>TYQYNMNFEKLGKCIIINNKNFDKVTGMGVRNGTDKDAEALFKCFRSLGFDVIVYNDCSCAKMQDLLKKASEEDHTNAACFACILLSHGEENVIYGKDGVTPIKDLTAHFRGDRCKTLLEKPKLFFIQACRGTELDDGIQADSGPINDTDANPRYKIPVEADFLFAYSTVPGYYSWRSPGRGSWFVQALCSILEEHGKDLEIMQIL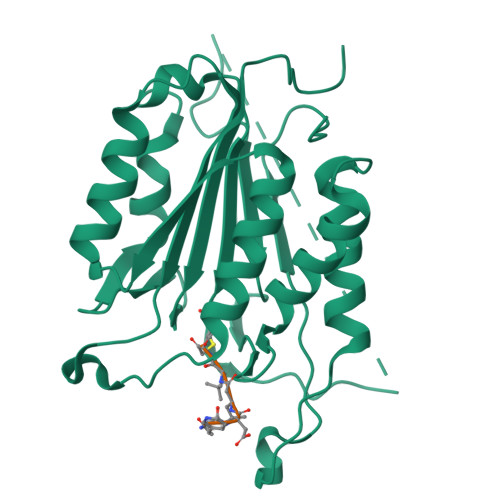TRVNDRVARHFESQSDDPHFHEKKQIPCVVSMLTKELYFSQQLHHHHHH[2x]>SMEDSMDMDMSPLRPQNYLFGCELKADKDYHFKVDNDENEHQLSLRTVSLGAGAKDELHIVEAEAMNYEGSPIKVTLATLKMSVQPTVSLGGFEITPPVVLRLKCGSGPVHISGQHLVAVEEDAESEDEEEEDVKLLSISGKRSAPGGGSKVPQKKVKLAADEDDDDDDEEDDDEDDDDDDFDDEEAEEKAPVKKSIRDTPAKNAQKSNQNGKDSKPSSTPRSKGQESFKKQEKTPKTPKGPSSV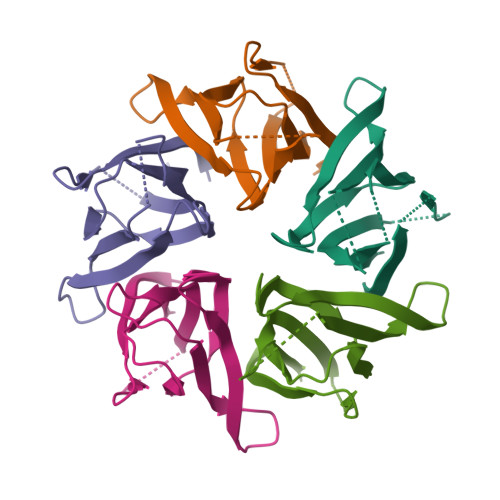EDIKAKMQASIEKGGSLPKVEAKFINYVKNCFRMTDQEAIQDLWQWRKSL[5x]> CPRMGHVFPLETRPYNQGSRLTAYELVYDKIPSTLITDSSIAYRIRTSPIPIKAAFVGADRIVRNGDTANKIGTLQLAVICKQFGIKFFVVAPKTTIDNVTETGDDIIVEERNPEEFKVVTG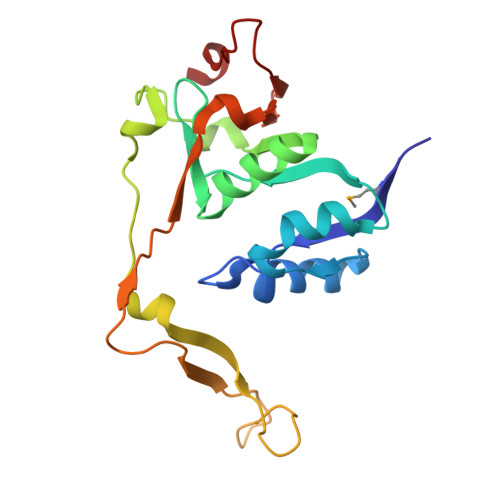TVINPENGSLILNESGEPITGKVGIAPLEINVWNPAFDITPHELIDGIITEEGVFTKNSSGEFQLESLF>[2x]MSRNCLDLYEEILTEEGTAKEATYNDLQVEYGKCQLQMKELMKKFKEIQAQNFSLINENQSLKKNISALIKTARVEINRKDEEISNLHLEHHHHHH

FLASH, Flice-associated huge protein, was originally discovered as a protein involved in Fas-mediated apoptosis and later in regulation of expression of several genes, including oncogenes. Subsequent studies showed that FLASH localizes to Histone Locus Bodies in the nucleus, suggesting a role in expression of histone genes, and that it is essential for histone pre-mRNA processing. Biochemical studies revealed that the interacting N-terminal regions of Lsm11 and FLASH form a docking platform that recruits the HCC to the U7 snRNP. Our crystallographic studies of FLASH NTD demonstrate that residues 71–137 adopt a continuous and stable α-helical fold and mediate the formation of a coiled-coil dimer between two FLASH molecules.

We determined a structure of the wild-type human FLASH NTD at 2.6 Å resolution using X-ray crystallography. The initial phases were obtained by the single anomalous dispersion (SAD) method using crystals of selenomethionyl FLASH NTD. The structure showed that FLASH NTD forms a coiled-coil dimer consisting of two parallel α-helices, one from each protomer. However, only residues 71 to 137 were observed in this structure, even though the expression construct contained residues 51–137. Residues 51–70, which include the LDLY motif previously shown to be essential for histone pre-mRNA processing and for binding the HCC, are disordered in this crystal. The length of the coiled-coil FLASH NTD dimer is approximately 100 Å, excluding the C-terminal hexahistidine tag observed for one of the protomers. The protomers do not superimpose perfectly onto each other (r.m.s.d. ~1.5 Å), and one of them appears to adopt a straighter conformation. Other hydrophobic interactions are formed by bulky residues such as Tyr73, Tyr80, and Phe94, as well as Met87 (selenomethionine in this structure). We also observed that Cys83 is situated in the dimer interface with the thiol side chains from the two protomers positioned near one another. While the electron density did not provide conclusive evidence for the existence of a disulfide bond, and the two sulfur atoms are separated by 3.4 Å distance in the current model, the structure raises the possibility that the observed FLASH NTD dimer might be mediated by a disulfide connection, which is unlikely to occur in the reducing environment in the nucleoplasm, the site of 3’-end processing.>MENSEKTEVVLLACGSFNPITNMHLRLFELAKDYMNGTGRYTVVKGIISPVGDAYKKKGLIPAYHRVIMAELATKNSKWVEVDTWESLQKEWKETLKVLRHHQEKLEASDCDHQQNSPTLERPGRKRKWTETQDSSQKKSLEPKTKAVPKVKLLCGADLLESFAVPNLWKSEDITQIVANYGLICVTRAGNDAQKFIYESDVLWKHRSNIHVVNEWIANDISSTKIRRALRRGQSIRYLVPDL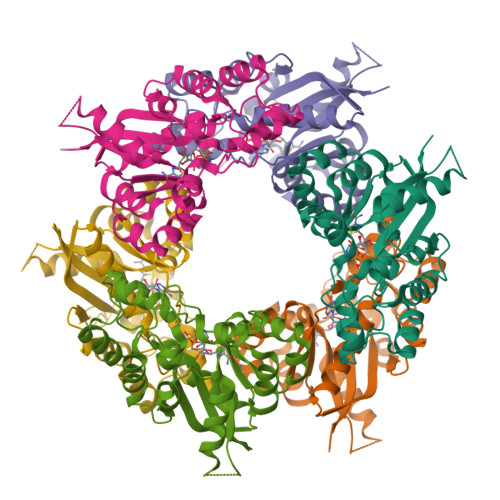VQEYIEKHNLYSSESEDRNAGVILAPLQRNTAEAKT[6x]Here, the structure of the novel tetracycline antibiotic TP-6076, bound to both the Acinetobacter drug efflux pump AdeJ and the ribosome from Acinetobacter baumannii, using single-particle cryo-electron microscopy (cryo-EM), is elucidated. TP-6076 is a fully synthetic tetracycline class antimicrobial agent. For tetracycline-based compounds, ribosome inhibition is achieved by direct interaction with the 30S subunit to block the binding of tRNA to the A site. The inner membrane component of the system, AdeJ, is responsible for drug recognition and powering substrate extrusion by utilizing proton motive force (PMF) as its energy source.

AdeJ assembles as a homotrimer and adopts the typical fold of a hydrophobe-amphiphile efflux (HAE)-RND pump. In the TP-6076-bound AdeJ trimer, each protomer occupies a distinct structural state forming an asymmetric trimer. Using three metrics for classification, the AdeJ–TP-6076 complex was determined to consist of binding, access, and extrusion protomers. An extra density was observed in the binding protomer of AdeJ deep within the periplasmic cleft. This density corresponds to the bound TP-6076 antibiotic at the distal pocket of the binding protomer. The binding of TP-6076 is largely stabilized by both aromatic and hydrophobic interactions. Particularly, F178 and F616 participate in π-π stacking interactions with rings A and C, respectively. Additionally, V139 and F611 interact with the trifluoromethyl group of ring D, while G179, V613, and F277 participate in alkyl-alkyl and π-alkyl interactions with the diethylamino group on ring A. A326, Y327, and F629 are also engaged in alkyl-alkyl and π-alkyl interactions with the pyrrolidine group of ring D. Electrostatic interactions between Q87 and Q176 and the carboxamide group on ring A of the tetracycline core further stabilize TP-6076 binding to the distal pocket of AdeJ. As Mg2+ is known to coordinate with tetracyclines in the ribosome, it is somewhat surprising that no Mg2+ ions were found to bind the TP-6076 drug in the AdeJ–TP-6076 structure. Surprisingly, in order to better accommodate the aminoethyl and trifluoromethyl ring modifications and the shorter pyrrolidine group, TP-6076 is flipped relative to Era in AdeJ.

>[3x]MAQFFIHRPIFAWVIALVIMLAGILTLTKMPIAQYPTIAPPTVTIAATYPGASAETVENTVTQIIEQQMNGLDGLRYISSNSAGNGQASIQLNFEQGVDPDIAQVQVQNKLQSATALLPEDVQRQGVTVTKSGASFLQVIAFYSPDNNLSDSDIKDYVNSSIKEPLSRVAGVGEVQVFGGSYAMRIWLDPAKLTSYQLTPSDIATALQAQNSQVAVGQLGGAPAVQGQVLNATVNAQSLLQTPEQFKNIFLKNTASGAEVRLKDVARVELGSDNYQFDSKFNGKPAAGLAIKIATGANALDTAEAVEQRLSELRKNYPTGLADKLAYDTTPFIRLSIESVVHTLIEAVILVFIVMFLFLQNWRATIIPTLAVPVVVLGTFAVINIFGFSINTLTMFAMVLAIGLLVDDAIVVVENVERVMSEDHTDPVTATSRSMQQISGALVGITSVLTAVFVPMAFFGGTTGVIYRQFSITLVTAMVLSLIVALTFTPALCATILKQHDPNKEPSNNIFARFFRSFNNGFDRMSHSYQNGVSRMLKGKIFSGVLYAVVVALLVFLFQKLPSSFLPEEDQGVVMTLVQLPPNATLDRTGKVIDTMTNFFMNEKDTVESIFTVSGFSFTGVGQNAGIGFVKLKDWSKRTTPETQIGSLIQRGMALNMIIKDASYVMPLQLPAMPELGVTAGFNLQLKDSSGQGHEKLIAARNTILGLASQDKRLVGVRPNGQEDTPQYQINVDQAQAGAMGVSIAEINNTMRIAWGGSYINDFVDRGRVKKVYVQGDAGSRMMPEDLNKWYVRNNKGEMVPFSAFATGEWTYGSPRLERYNGVSSVNIQGTPAPGVSSGDAMKAMEEIIGKLPSMGLQGFDYEWTGLSLEERESGAQAPFLYALSLLIVFLCLAALYESWSIPFSVLLVVPLGVIGAIVLTYLGMIIKGDPNLSNNIYFQVAIIAVIGLSAKNAILIVEFAKELQEKGEDLLDATLHAAKMRLRPIIMTTLAFGFGVLPLALSTGAGAGSQHSVGFGVLGGVLSATFLGIFFIPVFYVWIRSIFKYKPKTINTQEHKS> NLKKAQNNLLNSQIKDAVDATVSFYQTLTEKYGEKYSKMAQELADKSKGKKIGNVNEALAAFEKYKDVLNK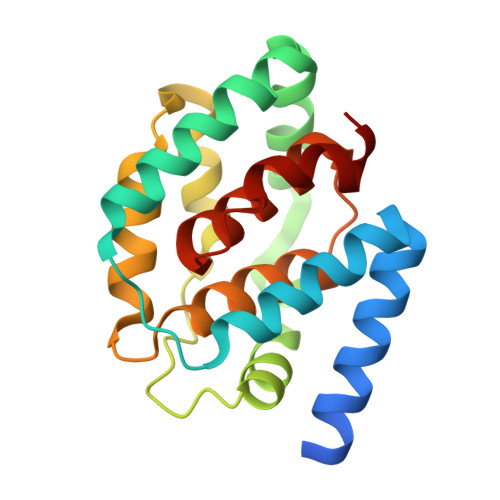KFSKADRDAIFNALASVKYDDWAKHLDQFAKYLKITGHVSFGYDVVSDILKIKDTGDWKPLFLTLEKKAADAGVSYVVALLFSLLAGTTLGIWGIAIVTGILCSYIDKNKLNTINEVLGI>[2x]MKNLTTIKQTNKNVKQERRKKYADLAIQGTNNSSIASKRSVELLYLPKLSSANNFQMDKNN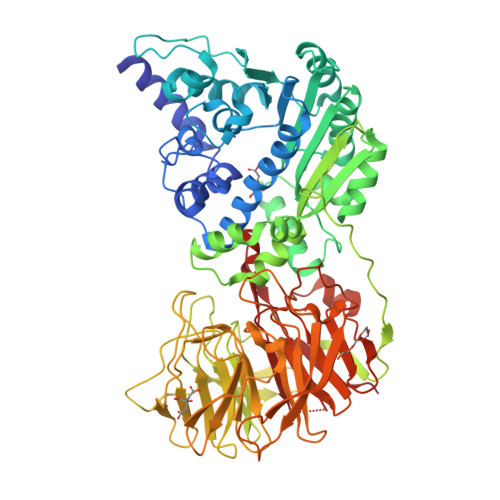KLLEYFKFFVPKKIKRSPCINRGYWLRLFAIRSRLNSIIEQTPQDKKIVVVNLGCGYDPLPFQLLDTNNIQSQQYHDRVSFIDIDYSDLLKIKIELIKTIPELSKIIGLSEDKDYVDDSNVDFLTTPKYLARPCDLNDSKMFSTLLNECQLYDPNVVKVFVAEVSLAYMKPERSDSIIEATSKMENSHFIILEQLIPKGPFEPFSKQMLAHFKRNDSPLQSVLKYNTIESQVQRFNKLGFAYVNVGDMFQLWESADEATKKELLKVEPFDELEEFHLFCHHYVLCHATNYKEFAFTQGFLFDRSISEINLTVDEDYQLLECECPINRKFGDVDVAGNDVFYMGGSNPYRVNEILQLSIHYDKIDMKNIEVSSSEVPVARMCHTFTTISRNNQLLLIGGRKAPHQGLSDNWIFDMKTREWSMIKSLSHTRFRHSACSLPDGNVLILGGVTEGPAMLLYNVTEEIFKDVTPKDEFFQNSLVSAGLEFDPVSKQGIILGGGFMDQTTVSDKAIIFKYDAENATEPITVIKKLQHPLFQRYGSQIKYITPRKLLIVGGTSPSGLFDRTNSIISLDPLSETLTSIPISRRIWEDHSLMLAGFSLVSTSMGTIHIIGGGATCYGFGSVTNVGLKLIAIAK(2~{S},4~{a}~{S},6~{a}~{R},6~{a}~{S},6~{b}~{R},8~{a}~{R},10~{S},12~{a}~{R},14~{b}~{R})-2,4~{a},6~{a},6~{b},9,9,12~{a}-heptamethyl-10-oxidanyl-13-oxidanylidene-3,4,5,6,6~{a},7,8,8~{a},10,11,12,14~{b}-dodecahydro-1~{H}-picene-2-carbothioic 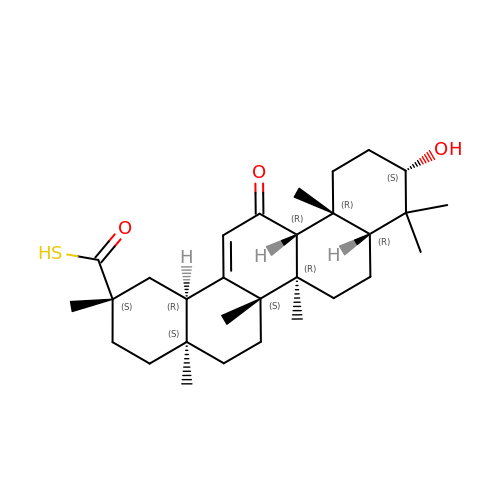S-acid | C30 H46 O3 S | SOGZTSGQAUOWBG-ZEYMVYSOSA-N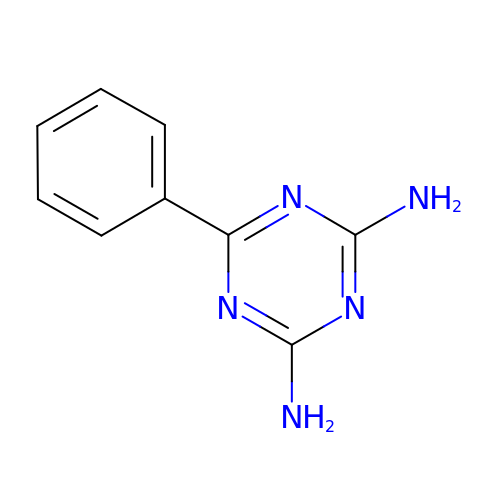6-phenyl-1,3,5-triazine-2,4-diamine | C9 H9 N5 | GZVHEAJQGPRDLQ-UHFFFAOYSA-N> GSHMTDPRKNGDLHEPATAPATPWSKSELVRQLRDLGVRSGDMVMPHVSLRAVGPLADGPQTLVDA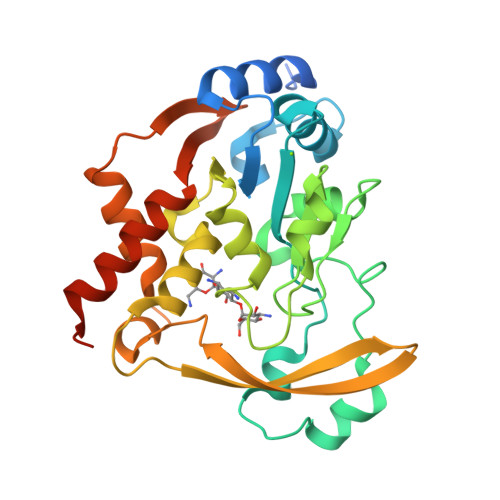LIEAVGPTGNILAFVSWRDSPYEQTLGHDAPPAAIAQSWPAFDPDHAPAYPGFGAINEFIRTYPGCRRSAHPDASMAAIGPDAAWLVAPHEMGAAYGPRSPIARFLAHAGKILSIGAGPDAVTALHYAEAVARIEGKRRVTYSMPLLREGKRVWVTTSDWDSNGILDEYAAPDGPDAVERIARDYLARTRVAQGPVGGAQSRLIDAADIVSFGIEWLEARHAAPAAAALKPKQRRD>[2x]MEQAPSEALQSLSVSDSQIPQSSNSTPQLSPEEKFKIVRSVGEECIQEDELLN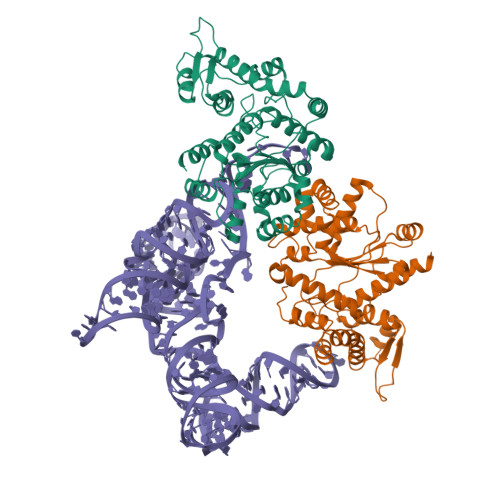LLTKKPEPVCYDGFEPSGRMHIAQGVMKTISVNKLTSAGCRVKIWIADWFAKLNNKMGGDLKKIETVGRYLIEIWKAVGMDVEGGKVEFLWSSKEINARADEYWPLVLDIAQKNNLKRIIRCSQIMGRSEQDELTAAQIFYPCMQCADIFFLKADICQLGMDQRKVNVLAREYCDDIKRKNKPIILSHHMLPGLQQGQEKMSKSDPSSSVFMEDEEAEVNVKIKKAYCPPKVVEGNPCLEYIKYLILPWFNEFTVERSADNGGNKTFKSYEELIADYESGELHPADLKPALSKSLNKILEPVREHFRKDSNAKELLKRVKAYRVTK The crystal structure of a CNT from Vibrio cholerae (vcCNT) presents the first opportunity to examine specific nucleoside recognition by CNTs from a structural perspective. vcCNT is an excellent model system to study hCNTs: it utilizes a Na+ gradient for nucleoside transport like hCNTs and shares high sequence identity (36–39%) with hCNTs with particularly high sequence identity for the nucleoside-binding site (64% with hCNT1, 73% with hCNT2, 91% with hCNT3). vcCNT forms a homotrimer with each protomer possessing its own nucleoside-binding site and permeation pathway. The protomer adopts a new fold and is divided into two domains: the scaffold domain that is responsible for trimerization and maintaining the overall architecture of the transporter (light blue), and the transport domain where nucleoside binding and transport occur (other colors). Two helical hairpins (HP1 and HP2) and two unwound helices (TM4 and TM7), related by twofold pseudo-symmetry, create a bowl-shaped nucleoside-binding site at the center of the transport domain of vcCNT.

The purine nucleoside adenosine and the antiviral guanosine analog ribavirin also possess similarly weaker binding affinity (KD = 470 and 1530 μM, respectively). To examine the structural basis of the reduced affinity, we solved the crystal structures of vcCNT-7C8C bound to adenosine and ribavirin. The structures reveal that the bulky purine base displaces the water observed in the uridine structure while maintaining similar modes of ribose binding, corroborating the idea that the reduced affinities of adenosine and ribavirin are due to the loss of the water-mediated interactions and highlighting the importance of the water coordinated by Thr 155 and Glu 156 in nucleoside recognition by CNTs.

> GPAVPRMSLFMSCCGMAVLLGIAVLLSSNRKAINLRTVGGAFAIQFSLGAFILYVPWGQELLRGFSDAVSNVINYGNDGTSFLFGGLVSGKMFEVFGGGGFIFAFRVLPTLIFFSALISVLYYLGVMQWVIRILGGGLQKALGTSRAESMSAAANIFVGQTEAPLVVRPFVPKMTQSELFAVMCGGLASIAGGVLAGYASMGVKIEYLVAASFMAAPGGLLFAKLMMPETEKPQDNEDITLDGGDDKPANVIDAAAGGASAGLQLALNVGAMLIAFIGLIALINGMLGGIGGWFGMPELKLEMLLGWLFAPLAFLIGVPWNEATVAGEFIGLKTVANEFVAYSQFAPYLTEAAPVVLSEKTKAIISFALCGFANLSSIAILLGGLGSLAPKRRGDIARMGVKAVIAGTLSNLMAATIAGFFLSF>SPNIKIFSGSSHQDLSQKIADRLGLELGKVVTKKFSNQETCVEIGESVRGEDVYIVQSGCGEINDNLMELLIMINACKIASASRVTAVIPCFPYARQDKKDKSRAPISAKLVANMLSVAGADHIITMDLHASQIQGFFDIPVDNLYAEPAVLKWIRENISEWRNCTIVSPDAGGAKRVTSIADRLNVDFALIHKERKKANEVDRMVLVGDVKDRVAILVDDMADTCGTICHAADKLLSAGATRVYAILTHGIFSGPAISRINNACFEAVVVTNTIPQEDKMKHCSKIQVIDISMILAEAIRRTHNGASVSY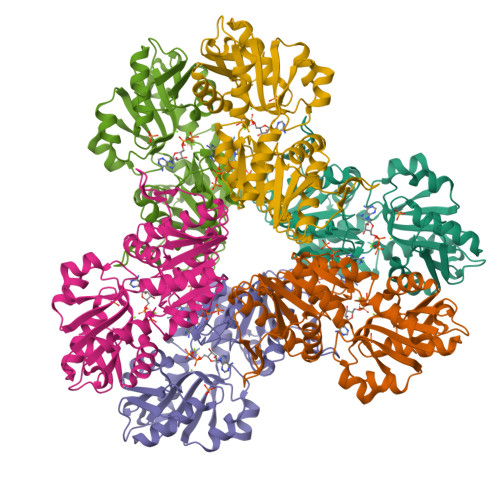LFSHVPL[6x]(2S)-2,6-diacetamido-N-methyl-hexanamide 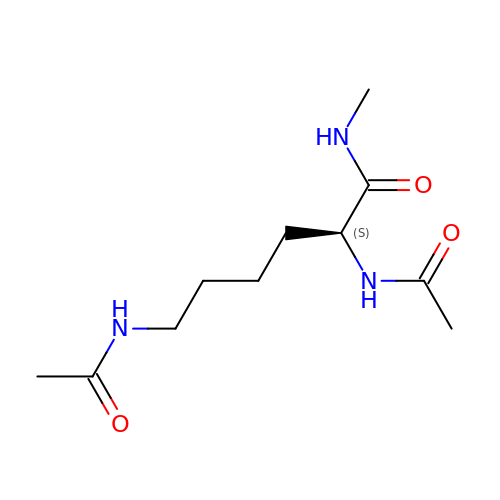| C11 H21 N3 O3 | RWBIXQSLRNBRKV-JTQLQIEISA-N> GTSTQTKAGSLTIVGTGIESIGQMTLQALSYIEAAAKVFYCVIDPATEAFILTKNKNCVDLYQYFDNGKSRLNTYTQMSELMVREVRKGLDVVGVFYGHPGVFVNPSHRALAIAKSEGYRARMLPGVSAEDCLFADLCIDPSNPGCLTYEASDFLIRDRPVSIHSHLVLFQVGCVGIADFNFTGFDNNKFGVLVDRLEQEYGAEHPVVHYIAAMMPHQDPVTDKYTVAQLREPEIAKRVGGVSTFYIPPKARKASNLDIIRRLELLPAGQVPDKKARIYPANQWEPDVPEVEPYRPSDQAAIAQLADHAPPEQYQPLATSKA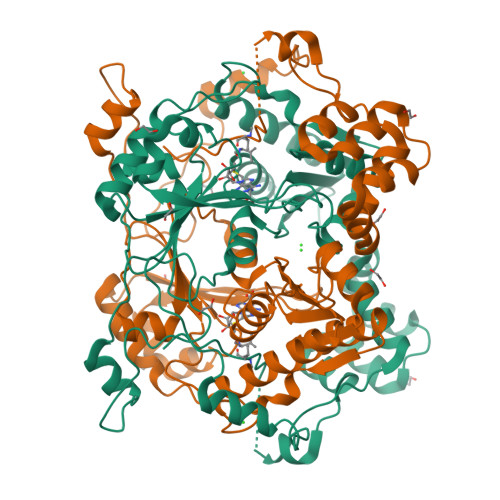MSDVMTKLALDPKALADYKADHRAFAQSVPDLTPQERAALELGDSWAIRCAMKNMPSSLLDAARESGEEASQNGFPWVIVVGVIGVIG>[2x]VLGKPQTDPTLEWFLSHCHIHKYPSKSTLIHQGEKAETLYYIVKGSVAVLIKDEE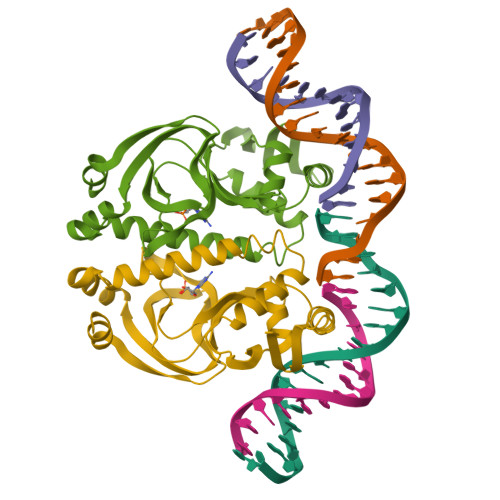GKEMILSYLNQGDFIGELGLFEEGQERSAWVRAKTACEVAEISYKKFRQLIQVNPDILMRLSAQMARRLQVTSEKVGNLAFLDVTGRIAQTLLNLAKQPDAMTHPDGMQIKITRQEIGQIVGCSRETVGRILKMLEDQNLISAHGKTIVV>[2x]PRLYFENRSKFIQDQKDKGINPYPHKFERTISIPEFIEKYKDLGNGEHLEDTILNITGRIMRVSASGQKLRFF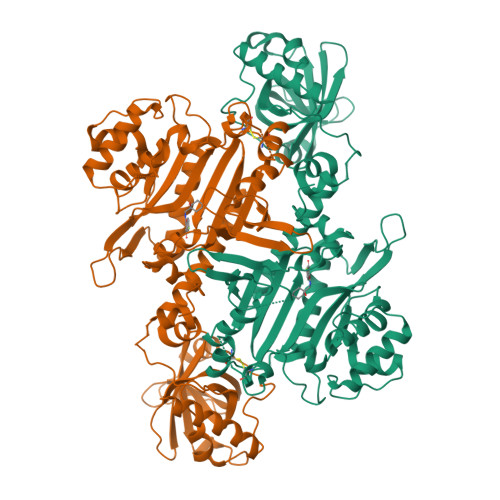DLVGDGEKIQVLANYSFHNHEKGNFAECYDKIRRGDIVGIVGFPGKSKKGELSIFPKETILLSACLHMLPMKYGLKDTEIRYRQRYLDLLINESSRHTFVTRTKIINFLRNFLNERGFFEVETPMMNLIAGGANARPFITHHNDLDLDLYLRIATELPLKMLIVGGIDKVYEIGKVFRNEGIDNTHNPEFTSCEFYWAYADYNDLIKWSEDFFSQLVYHLFGTYKISYNKDGPENQPIEIDFTPPYPKVSIVEEIEKVTNTILEQPFDSNETIEKMINIIKEHKIELPNPPTAAKLLDQLASHFIENKYNDKPFFIVEHPQIMSPLAKYHRTKPGLTERLEMFICGKEVLNAYTELNDPFKQKECFKLQQKDREKGDTEAAQLDSAFCTSLEYGLPPTGGLGLGIDRITMFLTNKNSIKDVILFPTMRPA> MPINRPNLNLNIPPLNIVAAYDGAEIPSTNKHLKNNFNSLHNQMRKMPVSHFKEALDVPDYSGMRQSGFFAMSQGFQLNNHGYDVFIHARRESPQSQGKFAGDKFHISVLRDMVPQAFQALSGLLFSEDSPVDKWAVTDMEKVVQQARVSLGA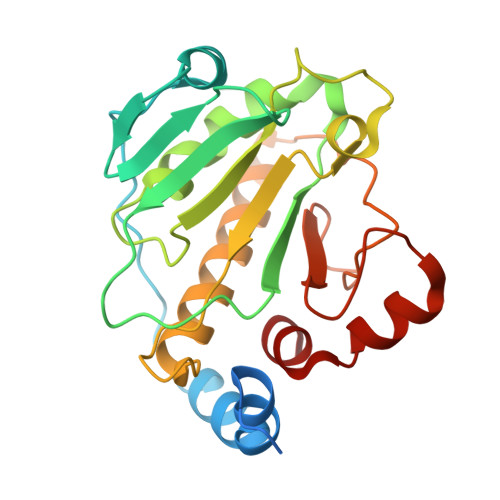QFTLYIKPDQENSQYSASFLHKTRQFIECLESRLSENGVISGQCPESDVHPENWKYLSYRNELRSGRDGGEMQRQALREEPFYRLMTE> MKKYTCTVCGYIYDPEDGDPDDGVNPGTDFKDIPDDWVC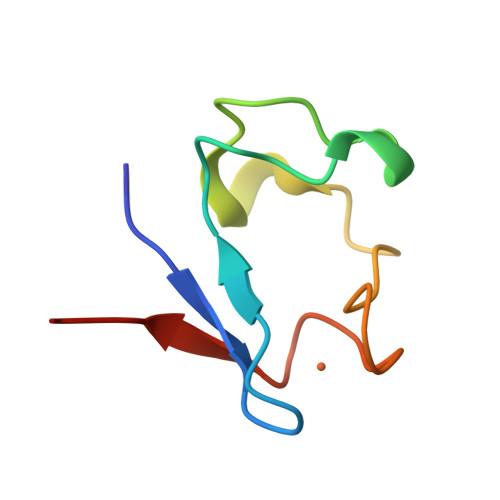PLCGVGKDEFEEVEE>[12x]MDKVYLTWWQVDRAIFALAEKLREYKPDVIIGVARGGLIPAVRLSHI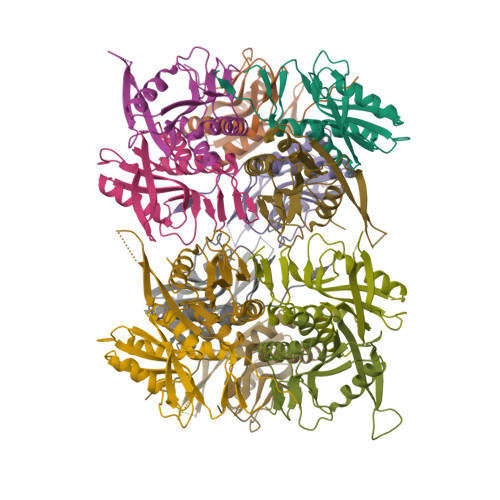LGDIPLKVIDVKFYKGIDERGEKPVITIPIHGDLKDKRVVIVDDVSDTGKTLEVVIEEVKKLGAKEIKIACLAMKPWTSVVPDYYVFRTEKWIVFPWEEFPVIEKE>MGVQTHVLELTSSVSAEKIFQGFVIDVD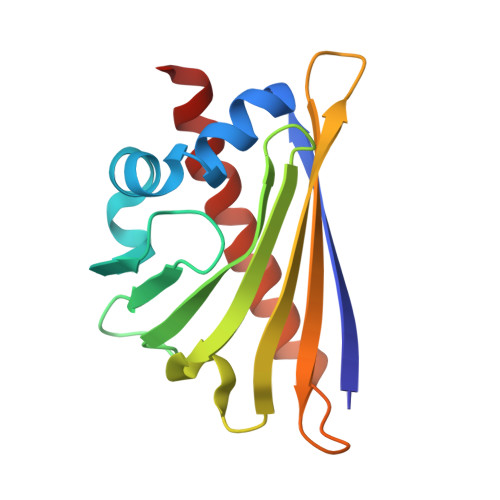TVLPKAAPGAYKSVEIKGDGGPGTLKIITLPDGGPITTMTLRIDGVNKEALTFDYSVIDGDILLGFIESIENHVVLVPTADGGSICKTTAIFHTKGDAVVPEENIKYANEQNTALFKALEAYLIAN[2x]>[2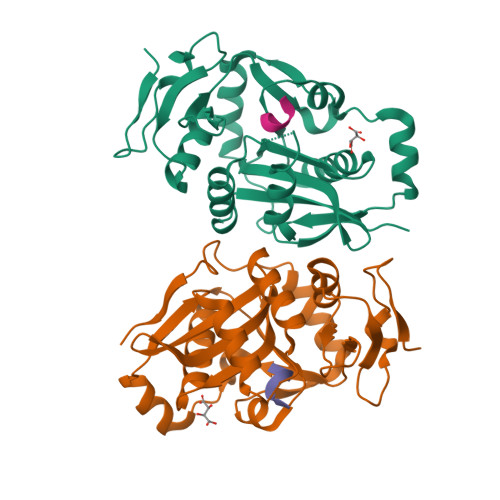x]RLVQLSRHSIAFPSPEGALREPNGLLALGGDLSPARLLMAYQRGIFPWFSPGDPILWWSPDPRAVLWPESLHISRSMKRFHKRSPYRVTMNYAFGQVIEGCASDREEGTWITRGVVEAYHRLHELGHAHSIEVWREDELVGGMYGVAQGTLFCGESMFSRMENASKTALLVFCEEFIGHGGKLIDCQVLNDHTASLGACEIPRRDYLNYLNQMRLGRLPNNFWVPRCLFSPQE;>FRYLG[2x]Human CEACAM1 (hCEACAM1) is a single pass type I transmembrane protein expressed as 12 alternatively spliced isoforms that all contain an N-terminal V set fold of the immunoglobulin superfamily (IgV) ectodomain followed by up to three type 2 constant immunoglobulin (IgC2) ectodomains (A1, B, A2), a transmembrane sequence, and a signaling cytoplasmic domain. CEACAM1 function is triggered by intercellular or trans binding of the IgV domain, resulting in higher order surface CEACAM1 oligomerization and subsequent intracellular signal transduction. In contrast to other immunoreceptors such as the T cell inhibitory and mucin domain-containing protein 3 (TIM-3), programmed cell death protein 1 (PD-1), and programmed death-ligand 1 (PD-L1), CEACAM1 serves as its own primary ligand, owing to high affinity homophilic interactions of its unique IgV domain, as well as an important microbial receptor. The displaced CC′ loop forms a cleft with the FG loop that exposes the key residues F29, S32, Y34, V39, G41, Q44, Q89, I91, N97, and E99 critical in mediating homophilic CEACAM1 interactions.

The E99A mutant structure revealed a GFCC′ face-mediated homodimer structure globally similar to the WT homodimer but with localized conformational differences resulting in a C-alpha root mean square deviation (RMSD) of 0.3 Å (over 1539 atoms). Interestingly, fewer hydrogen bonds (12 vs 17 for E99A and WT, respectively) and weaker hydrophobic interactions were observed for E99A homodimer. Specifically, side chain to main-chain backbone interactions between E99-G41 were abrogated and the intermolecular hydrogen bond network between residues Q89-Y34, N97-Y34, and Q89-N97 (using nomenclature convention here and after, where Q89 residue is from molecule (a) and Y34 residue in italics is from molecule (b) present in the crystal asymmetric unit) were disrupted at the E99A mutant homodimer interface. In addition, the distance between two opposing hydrophobic valine (V39) residues was slightly higher in the E99A homodimer (3.9 Å) compared to WT (3.7 Å). Similarly, we observed a CSS score of 0.63 for the E99A mutant, which demonstrated the presence of a slightly weakened GFCC′ face dimer. The I91A IgV domain adopts a GFCC′-mediated homodimer with RMSD of 0.6 Å (over 1489 atoms) compared to the WT homodimer with fewer hydrogen bonded (12 vs 17 for I99A and WT, respectively) and weaker hydrophobic interactions (specially for residue F29). Thus, the loss of important hydrogen bond interactions and possibly weaker hydrophobic interactions observed in the E99A and I91A mutant structure support the weak dimeric nature of these mutants as observed in our biophysical studies and previous reports.

>[2x]QLTTESMPFNVAEGKEVLLLVHNLPQQLFGYSWYKGERVDGNRQIVGYAIGTQQATPGPANSGRETIYPNASLLIQNVTQNDTGFYTLQVIKSDLVNEAATGQFHVY>MRVGLVGWRGMVGSVLMQR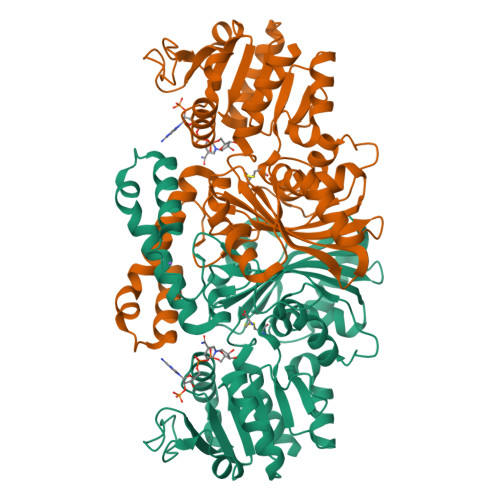MVEERDFDLIEPVFFSTSQIGVPAPNFGKDAGMLHDAFDIESLKQLDAVITCQGGSYTEKVYPALRQAGWKGYWIDAASTLRMDKEAIITLDPVNLKQILHGIHHGTKTFVGGNCTVSLMLMALGGLYERGLVEWMSAMTYQAASGAGAQNMRELISQMGVINDAVSSELANPASSILDIDKKVAETMRSGSFPTDNFGVPLAGSLIPWIDVKRDNGQSKEEWKAGVEANKILGLQDSPVPIDGTCVRIGAMRCHSQALTIKLKQNIPLDEIEEMIATHNDWVKVIPNERDITARELTPAKVTGTLSVPVGRLRKMAMGDDFLNAFTVGDQLLWGAAEPLRRTLRIILAEK[2x]>[4x]TETTSFSITKFGPDQQNLIFQGDGYTTKERLTLTKAVRNTVGRALYSSPIHIWDSKTGNVANFVTSFTFVIDAPNSYNVADGFTFFIAPVD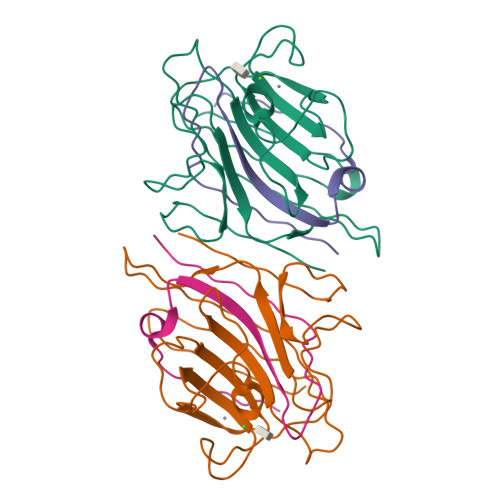TKPQTGGGYLGVFNSKDYDKTSQTVAVEFDTFYNTAWDPSNGDRHIGIDVNSIKSINTKSWALQNGKEANVVIAFNAATNVLTVSLTYPN;>[4x]ETSYTLNEVVPLKEFVPEWVRIGFSATTGAEFAAHEVLSWYFHSELAGTSSS> GSNSSTIAYSKSQHEAPKQLLQLRSEIKPLIPLNQ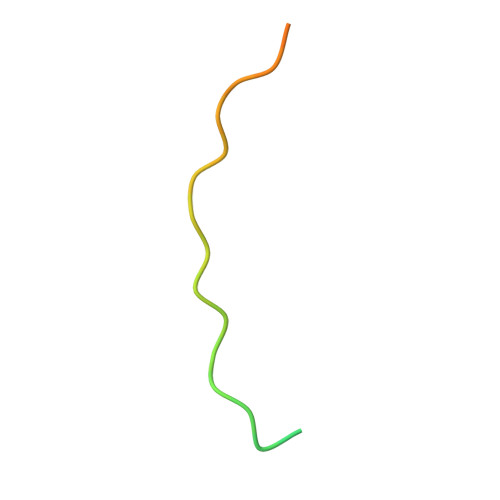P> MGSSHHHHHHSSGLVPRGSHMASSHAQTANWTEIYPGVWKATVGKPESYDLLKAAGAQPNKDALSKTEKVSFPFANGGVSLEVSGGKTYLRFPLQKEEQLYGFGLNFQTVHQRGKILELHVDHYGGKDSGRTHAPTPFYVSSNGYGVFINSARYIKVWAGTGVRKDSENFPTPKDRNTDKTWSSRPYSDAVEILVPAEGVEVYVFGGPKPIDAVKRYNLLNGGGYLPPRWGLGFTQRVMTRYTDKDVEKEVNDFKEKGYPLDFVGLEPGWQSKAYPGTFSWDKSRYPDPTSFVKKMKDQGIRLNLWINPYISPDAPFYKEIKPYTGSHTVWLGLVPDFTMAEARKPFFNQLLKDQIERGVSGYKIAEVDGYDYYLWPDAAKFPSGLSAEQMRQTYGLLVQRYSAELYKQRNERTFGLVRASNGGGTSFPYVIYNDYYNHQDFITALINSGF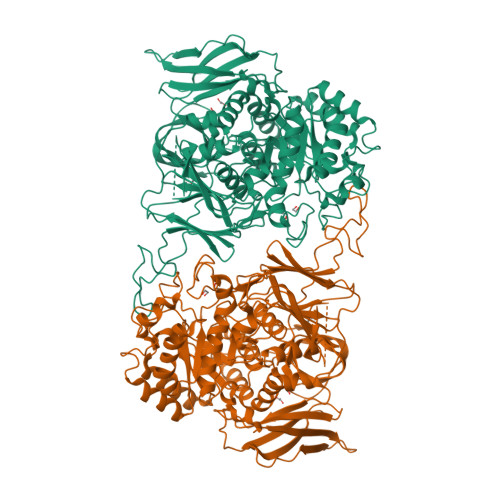AGVLWTPEVRASKSGEEWLRRFQSNVFSPMAMINAWASGTKPWSYPEVEADVKKFALLRMQMMPYWYSAFARYHFEGMPPFRGMGLEEGFRQDAKVEKLNKVNLEENPYAEAASKEIKDQYMAGDDLLVAPMFAGEKSRKVVLPKGKWYDFYTGEYAGDGEVLDVTPGLDKIPVYVRDGGIVPMMPALLNSPKSNQKVDLEIRYYGNKPGEFKLYDDDGETFNYEKGDFSWRTIRVEKDKSGKVKGSISAAVKGKVNTVGKVTFTAMTK>[2x]MAHHHHHHSAAL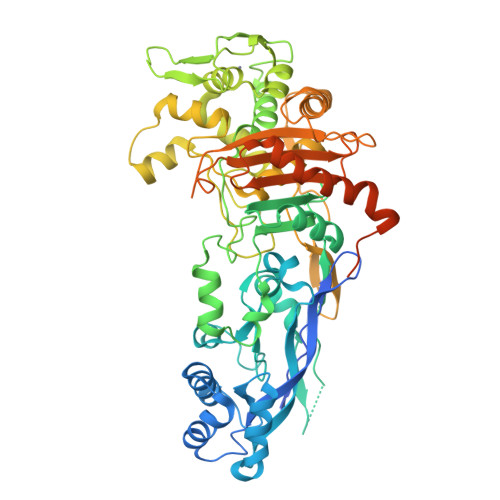EVLFQGPGYQASDKNRIRLQPLPPARGYIYDRNGVLLADNYPVFTATLSKADVENVDTVIEQLQPILELTQEDVDRFKSRIKTARKTERVAIKLNLTETNIAKFSEVKYKFPGVRIETQMTRYYPHGDLFAHVIGYVGRINDKELKSIDKDLYAGTNLIGKIGVEKSYEDLLHGTPGYESVEADAHSNILRHLGRKDPTRGNDLYLSLDYGLQVVASQQLAGRRGAIVAIDPRTGEILALVSSPSFNPNLFVTGINHKDYSSLRDNIDQPLYNRAVQGVYPPGSTIKPMEAMGGLHYGIVDWATAISDPGYFHLPGDSHKFRDWKKTGHGIVNMHKAIIMSCDTYFYILANQMGIDQMNQWMRQFGFGQKTGVDLPSESEGLYPNPEWKMRTRKSKWMKGETISVSIGQGAFTATPLQLAMATAITANHGSHVVPHVLRATHGAKPFTVRNAPDGKINFNGTDEDWVKMREAMIDVIQSGTGRGIRTPLYQIAGKTGTAQVKSIAQGKRYNEAALSERQLDHGLFVGFAPADKPEIAIAVIWENGRHGGSAAQLAKPVFDYWLLTRKKNPIRPANHQVNGGLMTAGIKPGELPSGNESASSTPATSAPTSAAASTPQATPTRPATNEVDE>GSHMGIEYRSLHTSQLTLSEKEALYDLLIEGFEGDFSHDDFAHTLGGMHVMAFDQQKLVGHVAIIQRHMALDNTPISVGYVEAMVVEQSYRRQGIGRQLMLQTNKIIASCYQLGLLSASDDGQKLYHSVGWQIWKGKLF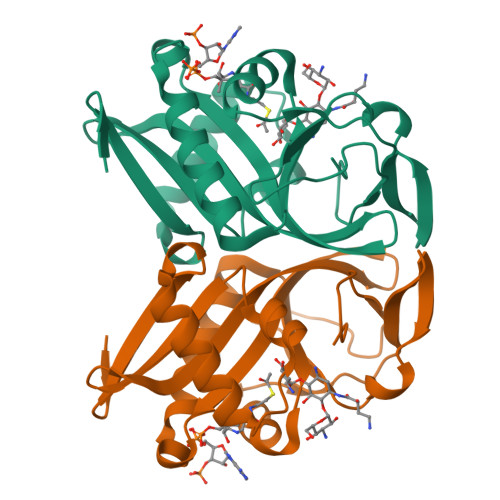ELKQGSYIRSIEEEGGVMGWKADGEVDFTASLYCDFRGGDQW[2x]> SGAIYVGNFRVVNRHLATHNDWANLVWEDSSRDLLVSSTTAQGCDTIARCNCQTGVYYCNSRRKHYPVSFSKPSLIYVEASEYYPARYQSHLMLAQGHSEPGDAGGILRCQHGVVGIVSTGGNG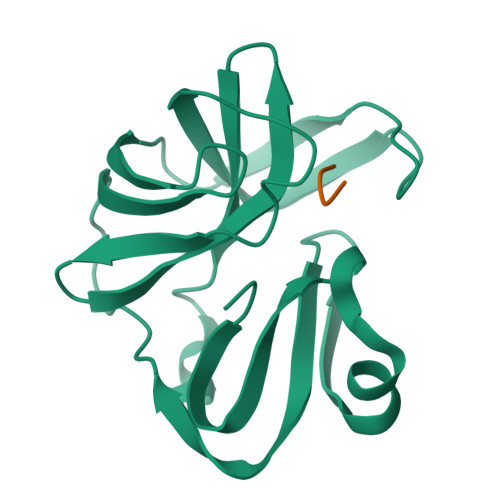LVGFADVRDLLWLD;> FRGK> KVFERCELARTLKRLGMDGYRGISLANWMCLAKWESGYNTRATNYNAGDRSTDYGIFQINSRYWCNDGKTPGA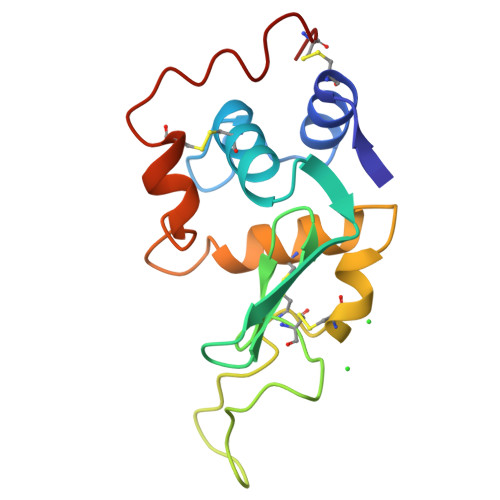VTGRGDSPANACHLSCSALLQDNIADAVACAKRVVRDPQGIRAWVAWRNRCQNRDVRQYVQGCGV> GPGSTTALQEALKEKQQHIEQLLAER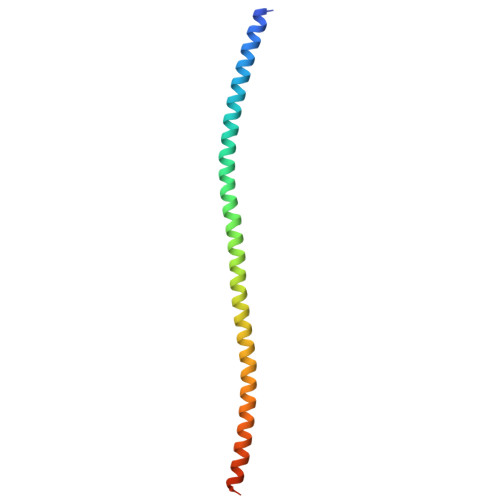DLERAEVAKATSHVGEIEQELALARDGHDQHVLELEAKMDQLRTMVEAADREKVELLNQLEEEKRKVEDLQFRVEEESITKGDLE> EFPEITEEMEKEIKNVFRNGNQDEVLSEAFRLTITRKDIQTLNHLNWLNDEIINFYMNMLMERSKEKGLPSVHAFNTFFFTKLKTAGYQAVKRWTKKVDVFSVDILLVPIHLGVHWCLAVVDFRKKNITYYDSMGGI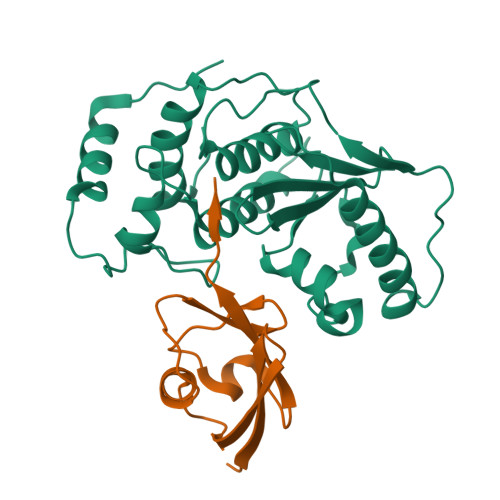NNEACRILLQYLKQESIDKKRKEFDTNGWQLFSKKSQIPQQMNGSDCGMFACKYADCITKDRPINFTQQHMPYFRKRMVWEILHRKLL;> NDHINLKVAGQDGSVVQFKIKRHTPLSKLMKAYCERQGLSMRQIRFRFDGQPINETDTPAQLEMEDEDTIDVFQQQTGG> AGYKTCPKVKPDMLNVHLVPHTHDDVGWLKTVDQYFYGIYNNIQPAGVQYILDSVISSLLANPTRRFIYVEIAFFSRWWRQQTNATQKIVRELVRQGRLEFANGGWVMNDEATTHYGAIIDQMTLGLRFLEETFGSDGRPRVAWHIDPFGHSREQASLFAQMGFDGFFFGRLDYQDKKVRKKTLQMEQVWRASTSLKPPTADLFTSVLPNMYNPPEGLCWDMLCADKPVVEDTRSPEYNAKELVRYFLKLATDQGKLYRTKHTVMTMGSDFQYENANTWFKNLDKLIQLVNAQQRANG;> IRVNVLYSTPACYLWELNKANLSWSVKKDDFFPYADGPYMFWTGYFSSRPALKRYERLSYNFLQVCNQLEALAGPAANVGPYGS;> GDSAPLNEAMAVLQHHDAVSGTSRQHVANDYARQLSEGWRPCEVLMSNALAHLSGLKEDFAFCRKLNISICPLTQTAERFQVIVYNPLGRKVDWMVRLPVSKHVYLVKDPGGKIVPSDVVTIPSSDSQELLFSALV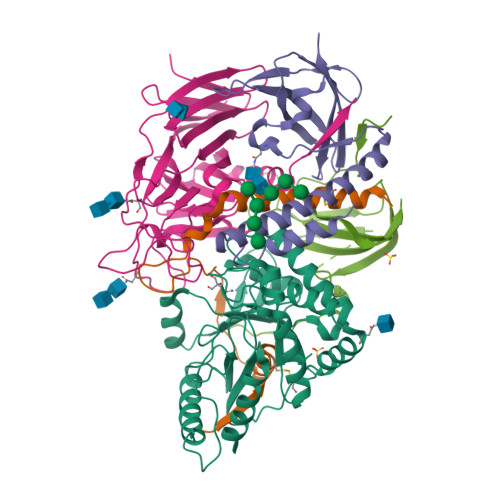PAVGFSIYSVSQMPNQRPQKSWS;> RDLVIQNEYLRARFDPNTGLLMELENLEQNLLLPVRQAFYWYNASTGNNLSSQASGAYIFRPNQNKPLFVSHWAQTHLVKASLVQEVHQNFSAWCSQVVRLYPRQRHLELEWTVGPIPVGDGWGKEVISRFDTALATRGLFYTDSNGREILERRRNYRPTWKLNQTEPVAGNYYPVNSRIYITDGNMQLTVLTDRSQGGSSLRDGSLELMVHRRLLKDDARGVGEPLNKEGSGLWVRGRHLVLLDKKETAAARHRLQAEMEVLAPQVVLAQGGGARYRLEKA;> PRTQFSGLRRELPPSVRLLTLARWGPETLLLRLEHQFAVGEDSGRNLSSPVTLDLTNLFSAFTITNLRETTLAANQLLAYASRLQWTTDTGPTPHPSPSRPVSATITLQPMEIRTFLASVQWEEDG> MGSSHHHHHHENLYFQSNAGPSIEVYVSAVSSPSRFWVQFVGPQVAQLDDLVAHMTEYYSKKENREAHTLRHVSVGQVVAAVFRHDGRWYRARVHDIRPNEFDSSQQVADVFYLDYGDSEYVATHELCELRADLLRLRFQAMECFLAGVRPASG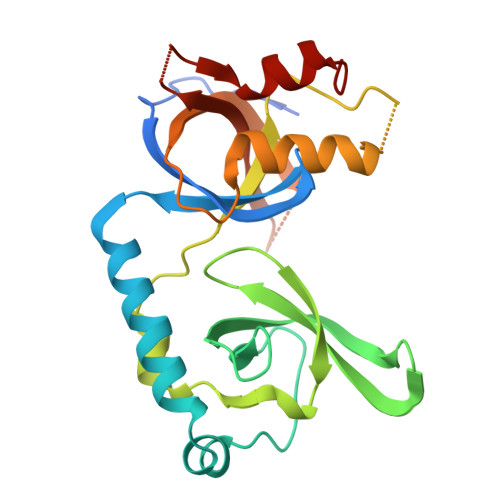EEAVSPSGQRWDKWHPQAVERFEELTQVARWKALVSRTCTYKKTATAEGEKDKEIPGIKLFDVTDEGELDVGAVLVAEGWAVA> MAFVSGAGAAVRGTSGKAAARCAAVRTVRAARAIRMTTAPGSAPFSSLDEPERQVVMWESVGDEKDQVFKQLYRQVFGNAYLMESDLEELLVPESQLLMGSISVKDFIKRVAKSDAYKKRFFE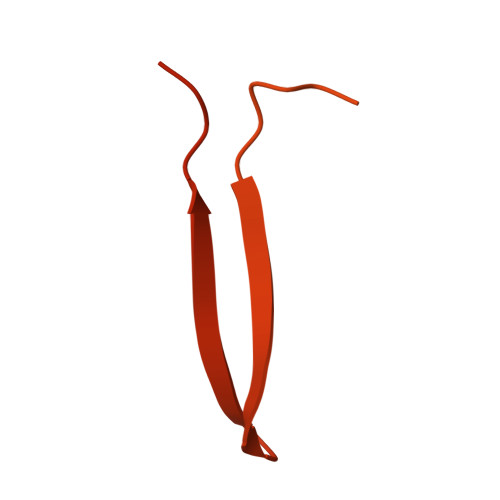PCGPYRFVELCTKHFLGRGPRDQKEVSEHVQRLANEGYDADVDSYMDSEEYMSLFGENGVPRFVFKGTYEGNDQFNRLAAMRQFADGSYTDTRSGSTAPRKAQKAELTMAEGDFVGRAKVSRGLPAETSAAKTGTPPVRALKGPVNPRAGVRVRIKVVDNLYQVYEIPPMADPKAKVNAFWAKPIPSSLTKKY>[2x]LP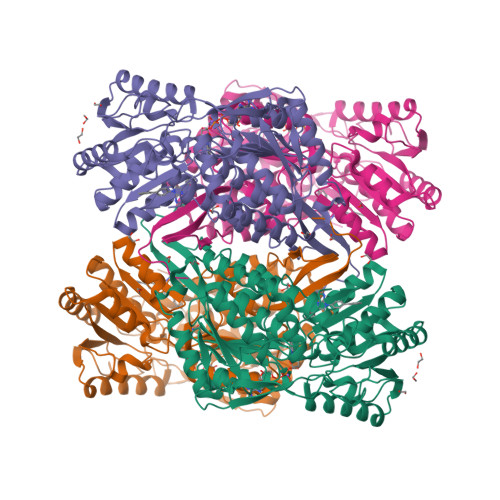SPILNPDIPYNQLFINNEWQDAVSKKTFPTVNPTTGEVIGHVAEGDRADVDRAVKAAREAFRLGSPWRRMDASERGRLLNRLADLVERDRVYLASLETLDNGKPFQESYALDLDEVIKVYRYFAGWADKWHGKTIPMDGQHFCFTRHEPVGVCGQIIPWNFPLVMQGWKLAPALATGNTVVMKVAEQTPLSALYLASLIKEAGFPPGVVNIITGYGPTAGAAIAQHMDVDKVAFTGSTEVGHLIQKAAGDSNLKRVTLELGGKSPSIVLADADMEHAVEQCHEALFFNMGQCCCAGSRTFVEESIYNEFLERTVEKAKQRKVGNPFELDTQQGPQVDKEQFERVLGYIQLGQKEGAKLLCGGERFGERGFFIKPTVFGGVQDDMRIAKEEIFGPVQPLFKFKKIEEVVERANNTRYGLAAAVFTRDLDKAMYFTQALQAGTVWVNTYNIVTCHTPFGGFKESGNGRELGEDGLKAYTEVKTVTIKVPQKNS> TQTSHPAKFHVEGEVYCNVCHSRNLINELSERMAGAQVQLDCKDDSKKVIYSIG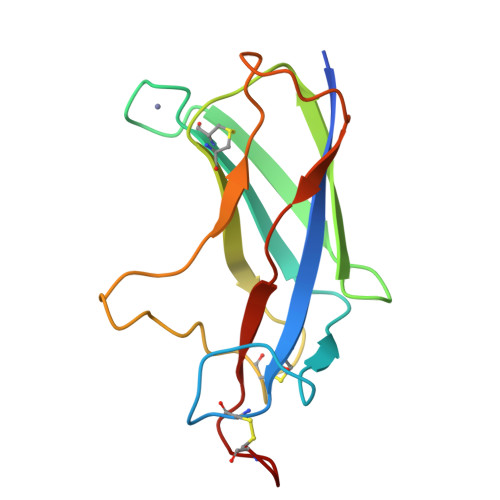GETDQDGVYRLPVVGYHEDCEIKLVKSSRPDCSEIPKLAKGTIQTSKVDLSKNTTITEKTRHVKPLSFRAKTDAPGC(2R)-2-azanyl-3-[[2-(4-methoxyphenyl)-2-tricyclo[9.4.0.0^{3,8}]pentadeca-1(11),3,5,7,12,14-hexaenyl]sulfanyl]propanoic acid | C25 H25 N 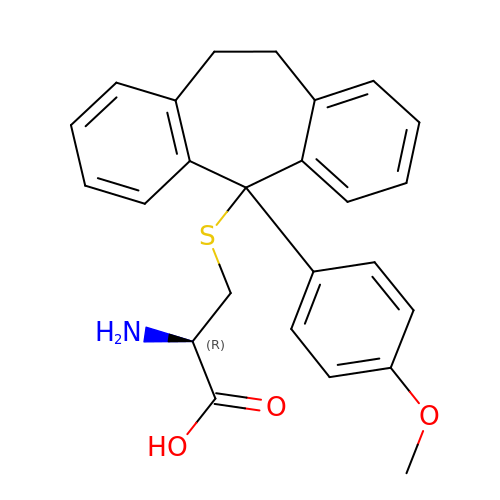O3 S | FFZDQAVDHIXOIW-QHCPKHFHSA-N> MKLLLFGYGNVGK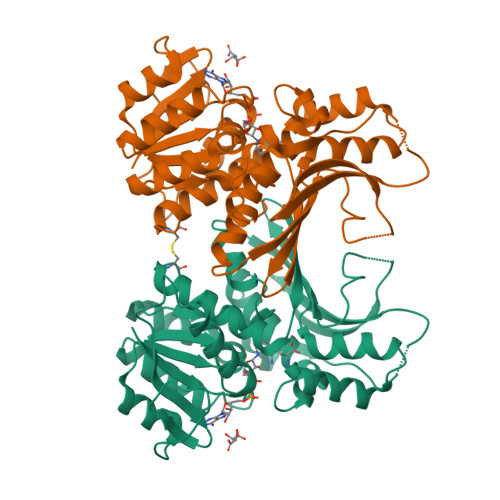AFRKLLHEKRSPELNDVIIGGIVTRRGIMLQDKEDFTPDLEGDVFKAFEKIKPDIIVDVSSANYNNGEPSLSLYKEAIKDGVNIITTNKAPLALAFNEIFSLARSKGVKIGFQGTVMSGTPSINLYRVLPGSRVIKIRGILNGTTNFILTLMNKGVSFEEALKEAQRRGYAEEDPTLDINGFDAAAKITILANFMIGNSVTIKDVKFEGINRDLPKNEKIKLIAYADEKEVWVKPLPISQDDPLYNVDGVENALEITTDIQSILIRGPGAGPVNAAYGALSDLILLKRDCL>GSKKKVKELKVLDSKTAQNLSIFLGSFRMPYQEIKNVILEVNEAVLTESMIQNLIKQMPEPEQLKMLSELKEEYDDLAESEQFGVVMGTVPRLRPRLNAILFKLQFSEQVENIKPEIVSVTAACEELRKSENFSSLLELTLLVGNYMNAGSRNAGAFGFNISFLCKLRDTKSADQKMTLLHFLAELCENDHPEVLKFPDELAHVEKASRVSAENLQKSLDQMKKQIADVERDVQNFPAATDEKDKFVEKMTSFVKDAQEQYNKLRMMHSNMETLYKELG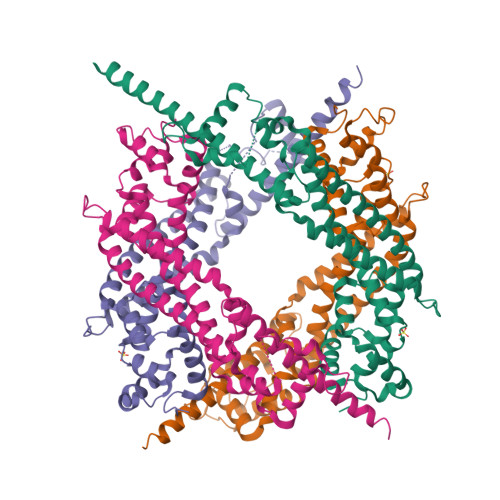DYFVFDPKKLSVEEFFMDLHNFRNMFLQAVKENQKRRETEEKMRRAKLAKEKAEKERLEKQ[4x]>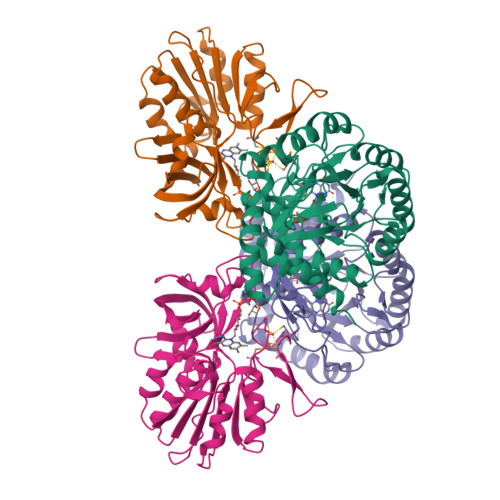 MTENNRLSVKLPGLDLKNPIIPASGCFGFGEEYAKYYDLNKLGSIMVKATTLHPRFGNPTPRVAETASGMLNAIGLQNPGLEVIMTEKLPWLNENFPELPIIANVAGSEEADYVAVCAKIGDAANVKAIELNISCPNVKHGGQAFGTDPEVAAALVKACKAVSKVPLYVKLSPNVTDIVPIAKAVEAAGADGLTMINTLMGVRFDLKTRQPILANITGGLSGPAIKPVALKLIHQVAQDVDIPIIGMGGVANAQDVLEMYMAGASAVAVGTANFADPFVCPKIIDKLPELMDQYRIESLESLIQEVKEGKK;> SQLQEMMTVVSQREVAYNIFEMVLKGTLVDEMDLPGQFLHLAVPNGAMLLRRPISISSWDKRAKTCTILYRIGDETTGTYKLSKLESGAKVDVMGPLGNGFPVAEVTSTDKILIIGGGIGVPPLYELAKQLEKTGCQMTILLGFASENVKILENEFSNLKNVTLKIATDDGSYGTKGHVGMLMNEIDFEVDALYTCGAPAMLKAVAKKYDQLERLYISMESRMACGIGACYACVEHDKEDESHALKVCEDGPVFLGKQLSL> MESKRNKPGK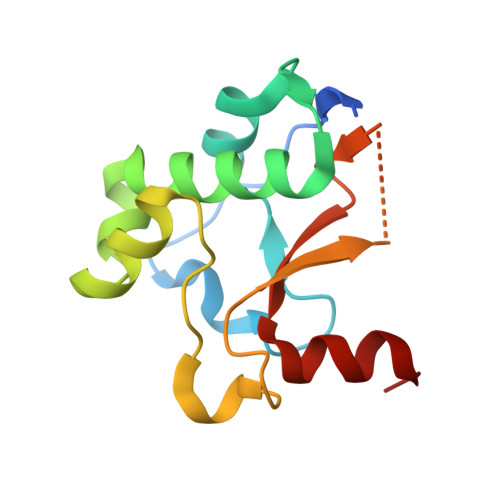ATGKGKPVNNKWLNNAGKDLGSPVPDRIANKLRDKEFKSFDDFRKKFWEEVSKDPELSKQFSRNNNDRMKVGKAPKTRTQDVSGKRTSFELHEEKPISQNGGVYDMDNISVVTPKRHIDIHRGK> INLSNKTDENTISFFDSGDPERMNSEALMRGCGEQIVNLRPLLRTFRTINDN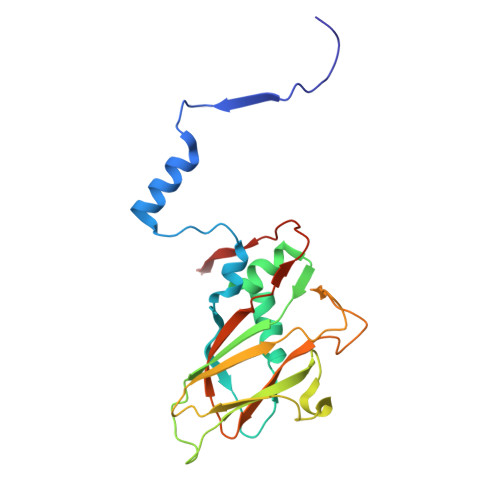WSLAANTKTPITDLTNTADAEGRDYMSYLSFLYRFYRGGRRYKFFNTTPLKQSQTCYVRSFLIPRNYTADEINTDGPSHITYPVINPVHEVEVPFYSQYRKIPIASTTDKGYDSSLMYYTNVGTQQIVARAGNDDFTFGWMIGTPQLQGITKEVAN>GSRQELQPWQRATYDFFMPQNLREDLQKKQFATLQVIPNSGLPQLEHWHSLVPLDTSNRKNTSCFGYPSWVYKAQNSRNGRHYALRRLEGYRLTNEKAILNVMKDWKKIKNASIVTIHEVFTTREFGDSSLIFAYDFHPLSKTLQEHHFQPIHGNRYRPPPAVPENTIWGYICQIANALKTIHSNRLAARCLEPSKIILTDINRIRLSACAILDVVQFGMNSRSVVELQQEDFVKFGKLILSLATGTLPAHLNNIPAALETLGNKYSANLKSAVNWLLDTSSGETKTIEHFMTGIASQMTTFFDLALQDNDEKLFHLAREVENGRIARSLMKLLTILERGDYDGVPSWSETGDRYQLKLFRDYVFHRVDADGKPNLSIGHMLTCMSKLEAGVDENILLTSRDNETVFVLSYRELRQMYDRAFNELVKASKTGAPGANT[4x];>[2x]GSMPLSSIGLPYYREPLFSAWPADIISDVGAPPLQLEPSFVATLKQAEWGLYGKNTRNVRRNQVEDTRNTNKQSNALQAPKFLSERARESALSSGGDSSSDPQVDQEPEDPNEIESLKP

Two conserved complexes carry out the majority of deadenylation in the cytoplasm: Pan2–Pan3 and Ccr4–Not. As illustrated in Fig1A, Pan3 contains a zinc finger at its N-terminus, a pseudokinase domain (PK), a coiled coil and a highly conserved C-terminal domain (CTD) (Brown et al, 1996; Christie et al, 2013; Wolf & Passmore, 2014). Pan2 contains three functional domains: an N-terminal WD40 domain, an inactive ubiquitin C-terminal hydrolase (UCH) domain and a C-terminal exonuclease (Fig1A) (Boeck et al, 1996; Wolf & Passmore, 2014). In conclusion, through combined biochemical and structural approaches, we have shown that Pan3 is required to couple RNA binding to the Pan2 exonuclease activity.

The best diffracting crystals were obtained with a construct that lacks the first 27 residues of the PID region, ctPan2343–458, had P21 symmetry and diffracted to 2.6 Å resolution with two copies of the complex in the asymmetric unit. Molecular replacement using the structure of ctPan3 PKC showed clear difference density corresponding to a single ctPan2 chain (comprising residues 355–406) on each ctPan3 dimer. The overall structure of the ctPan3 dimer in the complex closely resembled that obtained for ctPan3 alone (Cα RMSD 0.94 Å), although there was a slight (˜6°) rotation of the C-terminal domain relative to the coiled-coil and pseudokinase domain (Fig5C and D and Supplementary Fig S6C). The major difference between free and Pan2-associated ctPan3 was a substantial rotation of the N-terminus of chain B (residues 207–224) by approximately 90° toward the Pan3 CTD (Fig5C and D). The PID of ctPan2 exploits the asymmetry of the ctPan3 dimer by wrapping around it at the interface between the pseudokinase and C-terminal domain (Fig6). In particular, ctPan2 Phe357 and Trp360 are inserted into a pocket of ctPan3 formed by the C-terminal domain of chain A and the coiled coil (Fig6C). The PID of ctPan2 next passes over the coiled coil and interacts with the N-terminus of ctPan3 chain B (Gln212–Ala214) through an intermolecular antiparallel β-sheet (Fig6E). This new β-sheet is located between the pseudokinase domain of chain A and the CTD of chain B. The PID continues around Pan3 to form extensive interactions with the CTD of chain B that include an extended 4-strand antiparallel β-sheet between a β-hairpin of the ctPan2-PID (residues 384–393) and a β-hairpin ‘ear’ in ctPan3 (residues 597–612) (Fig6A). Finally, residues 399–403 of the PID of ctPan2 bind in a highly conserved groove formed by residues 599–603 and 562–573 in the CTD of chain B of the Pan3 dimer (Fig6D). Collectively, the interface between the PID of ctPan2 and the ctPan3 PKC dimer buries a surface area of approximately 2,230 Å2, and the ctPan3 PKC dimer interface buries approximately 3,740 Å2.>[2x]MPDEEKLQKYLRKVTAELQQARRRLAAAESQSQEPIAVLGIGCRFPGGVRSPEDLWDLVDSGGDAVGGLPAGRGWQAGSALDGVNAGFIHGVEEFDPYFFGLDPVEAAAMDPQQRLLLETTWEAFERAGIDPVAARGSRTAVYAGVQFGGYPLLMREAPPPQVLDHLGLGNSVGAASGRLAYQFGLLGGAVTVDTQCTSSIVALHLAVKALRNGECALALAGGACVMSLPTVLMDFHRRSLLAPDGRSKSFA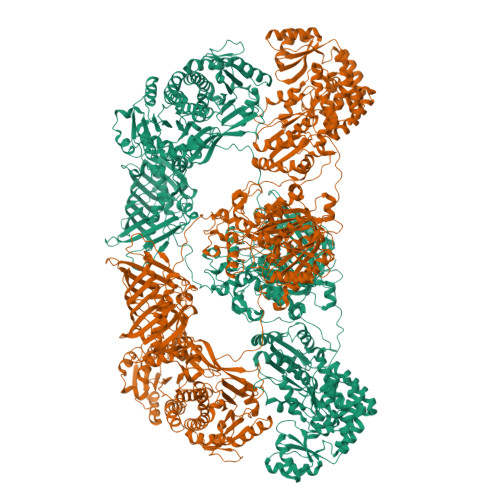AAADGVSLAEGAGMLLLERLSDARRNGHPVMAVIRGTAINQDGATNGIISPSGRAQERVIRAALADGRVTADSVDAVEGHGVGATLGDGVEVTSLLSTYGQERPAGRPLLLGSVKSNIGHTQTVGAVAGIVKLVMALRNERLPRTVHVDGPTPHADWSSGTVRLLTEPEPWRRGERVRRAGLTCLTLSGTNGHLILEEPPADEPAARPANPERTVPLVLSAKSPTALREQAERLRATITAAEPVDVGHSLHTTRSSFRHRAVVLGTGREELAAGLDALAGDRTADGLVRGVARAQGQTALLFGGAGDGTSGDRPADAEGPRTARGLYEAFPAFAEALDEVTEHLAGLLGPEVRAAVREPGPACAEPTVVGQAVAFALNTALHRLLTAFAVRPDATLGHGAGEVAAAYAAGALSLADGAALVTALGRITERVATGPGASVWVRATEDEVRAALSGSQEQVGAAVAAVDEPGTTVVSGDAGAVARVAAHWRAHGRATGAPRPARLLLSPDDEQAALAELRAIVAGLAFREPEVPLLSTVTGQPVEPAELRSAEHWLDHLRGPTRFLDGVRRLRTDGVTRLVGLDLSGDLTGPAGRSAAGFGEPGRPLLLASVPGGGRPPGQALLSALGELHTDGVAIDWSQAFEGRGARRVDLPTYPYQKVRCWLVPPEPQVSVVAAPPHPLLGTALDLVDATGQSFTQQLTPGQVAGVFGQQLYGTPVLPAGARLEWLLAAARHGSPDSAWTLTGIRLPGTVSAASGTPVALQTSREDSGDGHRVRAFVKGPGTGGGRWAERGGATVVPAVTRPAPDRVDPESLPEGLAELDVAEVYRRLWRQGSDYAEPLRVLRRVWLGGDEAVALVGTADVPTGPSGWSRWAAVLEAAVQLAALSGSGPRTPVSVDRLEVSGPPSEVVWLRVRHGADGAADAVVLSGEGVRLAAVQGLRLRPMAGREPAGLAEAPLERHEVVWHALAEDGRPGAIGGGTGSWLVFSDDPERAAAWCDELALFGVPAVALAGEDAEGRDGTETVPVGTGDPDVVGKTFAELRERGVTVAGLLVHDAGDAREPASGADDPLDAACRRGGRTLALVRGFLQEYAEQTPRIVLCSAGAAAGLAGGPPHPAQAPLTALFTSLVWEHPELPCAQVDLDPAEDPPTVVSLLGQVMRLPGAGRLAVRGGRWFEARLERRPAPADRGERLALRPDATYLVAGGDTRHAAAALEWLAARGARSVVLAGAESERGDLAGARTTGHAGIERLEHVAVDLSSAADVARLAELCADGRPPLRGVLLLPQPVAGGGLDELDGARFGAELAGALRGPVELTRRFTDVGLTGGTDFFVLSTSVVSLPGRAGTVVGSAADAFLTALARHHRQAGLPVVAAAWGPWLESVDESDEAPAVAFAEAGVYPAPGGEMLDALLPLPAAGEADGSGEAGLARVDWDRYLTAGHRPLPYTVLETRASYDEEKAPGFGQNRM> MLGVCYYPEHWPKERWKEDARRMREAGLSHVRIGEFAWALLEPEPGRLEWGWLDEAIATLAAEGLKVVLGTPTATPPKWLVDRYPEILPVDREGRRRRFGGRRHYCFSSPVYREEARRIVTLLAERYGGLEAVAGFQTDNEYGCHDTVRCYCPRCQEAFRGWLEARYGTIEALNEAWGTAFWSQRYRSFAEVELPHLTVAEPNPSHLLDYYRFASDQVRAFNRLQVEILRAHAPGKFVTHNFMGFFTDLDAFALAQDLDFASWDSYPLGFTDLMPLPPEEKLRYARTGHPDVAAFHHDLYRGVGRGRFWVMEQQPGPVNWAPHNPSPAPGMVRLWTWEALAHGAEVVSYFRWRQAPFAQEQMHAGLHRPDSAPDQGFFEAKRVAEELAALALPPVAQAPVALVFDYEAAWIYEVQPQGAEWSYLGLVYLFYSALRRLGLDVDVVPPGASLRGYAFAVVPSLPIVR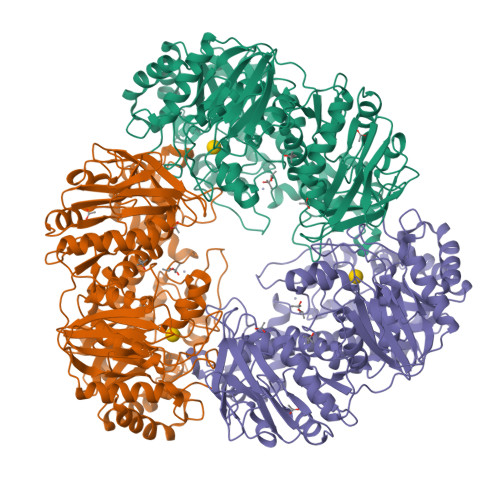EEALEAFREAEGPVLFGPRSGSKTETFQIPKELPPGPLQALLPLKVVRVESLPPGLLEVAEGALGRFPLGLWREWVEAPLKPLLTFQDGKGALYREGRYLYLAAWPSPELAGRLLSALAAEAGLKVLSLPEGLRLRRRGTWVFAFNYGPEAVEAPASEGARFLLGSRRVGPYDLAVWEEA2-(4-chloranylphenoxy)-~{N}-[4-[2-(4-chloranylphenoxy)ethanoylamino]cyclohexyl]ethanamide 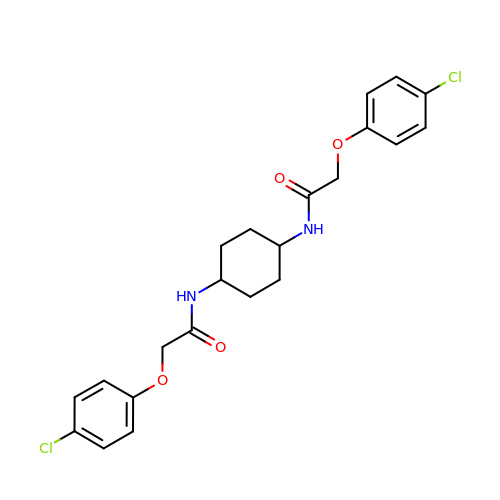| C22 H24 Cl2 N2 O4 | HJGMCDHQPXTGAV-IYARVYRRSA-N>MGSSHHHHHHSSGDHRKIGRDQELYFFHELSPGSCFFLPKGAYIYNALIEFIRSEYRKRGFQEVVTPNIFNSRLWMTSGHWQHYSENMFSFEVEKELFALKPMNCPGHCLMFDHRPRSWRELPLRLADFGVLHRNELSGALTGLTRVRRFQQDDAHIFCAMEQIEDEIKGCLDFLRTVYSVFGFSFKLNLSTRPEKFLGDIEVWDQAEKQLENSLNEFGEKWELNSGDGAFYGPKIDIQIKDAIGRYHQCATIQLDFQLPIRFNLTYVSHDGDDKKRPVIVHRAILGSVERMIAILTENYGGKWPFWLSPRQVMVVPVGPTCDEYAQKVRQQFHDAKFMADIDLDPGCTLNKKIRNAQLAQYNFILVVGEKEKISGTVNIRTRDNKVHGERTISETIERLQQLKEFRSKQAEEEF[4x]

ThrRS is one of the 20 (in general) aminoacyl-tRNA synthetases (AARSs) that are essential enzymes responsible for charging corresponding amino acids to their cognate tRNAs and providing the correct substrates for high-fidelity protein synthesis. We determined the crystal structures of both human and E. coli ThrRS in complex with BN, and identified a unique structural inhibition mechanism of BN against ThrRS. BN occupies a significant fraction of the total volume of the ThrRS enzymatic pocket, physically excluding all three of the physiological substrates of ThrRS, namely L-threonine (L-Thr), ATP and tRNA. Although occupying the canonical active site cavity, BN also extends into a fourth ‘orthogonal’ pocket.

To elucidate the species-independent, full-spectrum inhibitory mechanism of BN, we co-crystallized a fragment of human ThrRS containing the essential catalytic domain and anticodon-binding domain (residues 322–723) with BN and determined the structure to a resolution of 2.6 Å. As a typical class II AARS21, human ThrRS forms a dimer through the catalytic domain, with each subunit binding one molecule of BN. The polyketide BN binds tightly in the aminoacylation active site cavity of human ThrRS, constituted by class II AARS signature motif 2 (residue 432–469), motif 3 (585–613)22 and surrounding hydrophobic loops 386–393, 411–413, 538–540 and 564–567. The plane of the 18-membered ring in BN fits perpendicularly to the seven-stranded β-sheet of the catalytic domain. For instance, Q460 on the floor of motif 2 in human ThrRS forms a key hydrogen bond with the only carboxylic group of BN. Notably, the carboxyl acid group on BN precludes a key interaction in aminoacylation by forming a bifurcated salt-bridge with R442. By interacting with the guanidine group of R442, BN prevents R442 binding to L-Thr and ATP, thereby blocking the formation of the threonyl-adenylate (Thr-AMP). C4–5 of BN further pushes Y392 into the tRNAThr A76 adenosine-binding pocket, whereas in the tRNA-bound structure of the E. coli ThrRS, the corresponding Y313 stacks with the adenine ring of A76 for aminoacylation. In our structures, a major feature of the BN-induced conformational change is a 14° rotation of the α helix comprised by residues 431–448 that produce a 10-Å displacement of the preceding loop. This structural change is observed in both the human and E. coli ThrRS–BN complexes.>MYAPAAEDEHTITNWSGTHAVRPKRFFQPESVEELEKIVKEAHEKGQKIRPVGSGLSPNGLAFSEDGMVSLALMDKVLHVDKEKKQVTVQAGARVQQVVDALRPHGLTLQNFASISEQQIGGFIQVGAHGTGARIPPVDEQVVSMKLVTPAKGTIELSEEKDPELFRLARCGLGALGVVTEVTLQCVPRHKLLEHTFVATMKEVKKNHEKLLRENKHVRYMWIPYTDTVVVVTCNPLPEGKKAPKVKPQYSEDEKLQPLRNLLREAAPPARAPEVAAPSSSETSPEVSGLSFTELRDALLAVDPLDTEWVKRVNQAEAEFWKRSEGYRVGWSDEILGFDCGGQQWVSEVAFPAGTLEKPSAADLEYMEELMRLINKEGIPAPAPIEQRWTAGSSSPMSPAYSPSPDSVFSWVGIIMYLPTEDEEQRKAITEAFRQYRKLCETRLWDKYGAAEHWAKIEVPEDPEELEALRERLRKRYPGVDKFNKARRELDPKNILSNDMIDSLFPAAESA[3x]

In photosynthetic organisms, L-ascorbic acid is produced in the Smirnoff-Wheeler pathway by the multi-step conversion of D-mannose-6-phosphate to L-galactono-1,4-lactone, the substrate for the final biosynthetic enzyme, L-galactono-1,4-lactone dehydrogenase (GalDH) [EC 1.3.2.3]9,15. GULO, ALO, and GalDH are generally named aldonolactone oxidoreductases and form a group of sequence-related flavoenzymes belonging to the vanillyl-alcohol oxidase family. They oxidize the C2 carbon atom of their monosaccharide substrates and thereby generate the characteristic, redox-reactive C2-C3 double bond of L-ascorbic acid and its analogs. GalDH is a dehydrogenase that reacts poorly with oxygen.

To elucidate the structural features of GalDH and how it interacts with its substrate, we determined the crystal structures of the viridiplantae ancestor without (1.9 Å resolution) and with L-galactono-1,4-lactone (2.1 Å resolution). As a member of the vanillyl-alcohol oxidase family, the structure of vGalDH can be divided into flavin- (residues 1-189, 452-511) and substrate-binding (190-451) domains. The FAD is embedded in the flavin domain with the isoalloxazine ring in the classical position at the domain interface where an open cleft forms the active site on the si side of the flavin. For all three substrates, we observed only marginal oxidase activities (< 0.2 s−1). With the GalDH crystal structure at hand, we noticed that Ala113 is in direct contact with the N5-C4a locus of the flavin at the edge of the cofactor ring.>MAAAGASRLLERLLPRHDDFARRHIGPGDKDQREMLQTLGLASIDELIEKTVPANIRLKRPLKMEDPVCENEILATLHAISSKNQIWRSYIGMGYYNCSVPQTILRNLLENSGWITQYTPYQPEVSQGRLESLLNYQTMVCDITGLDMANASLLDEGTAAAEALQLCYRHNKRRKFLVDPRCHPQTIAVVQTRAKYTGVLTELKLPCEMDFSGKDVSGVLFQYPDTEGKVEDFTELVERAHQSGSLACCATDLLALCILRPPGEFGVDIALGSSQRFGVPLGYGGPHAAFFAVRESLVRMMPGRMVGVTRDATGKEVYRLALQTREQHIRRDKATSNICTAQALLANMAAMFAIYHGSHGLEHIARRVHNATLILSEGLKRAGHQLQHDLFFDTLKIQCGCSVKEVLGRAAQRQINFRLFEDGTLGISLDETVNEKDLDDLLWIFGCESSAELVAESMGEECRGIPGSVFKRTSPFLTHQVFNSYHSETNIVRYMKKLENKDISLVHSMIPLGSCTMKLNSSSELAPITWKEFANIHPFVPLDQAQGYQQLFRELEKDLCELTGYDQVCFQPNSGAQGEYAGLATIRAYLNQKGEGHRTVCLIPKSAHGTN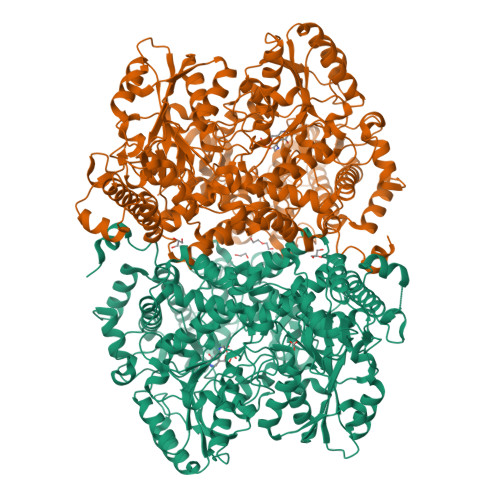PASAHMAGMKIQPVEVDKYGNIDAVHLKAMVDKHKENLAAIMITYPSTNGVFEENISDVCDLIHQHGGQVYLDGANMNAQVGICRPGDFGSDVSHLNLHKTFCIPHGGGGPGMGPIGVKKHLAPFLPNHPVISLKRNEDACPVGTVSAAPWGSSSILPISWAYIKMMGGKGLKQATETAILNANYMAKRLETHYRILFRGARGYVGHEFILDTRPFKKSANIEAVDVAKRLQDYGFHAPTMSWPVAGTLMVEPTESEDKAELDRFCDAMISIRQEIADIEEGRIDPRVNPLKMSPHSLTCVTSSHWDRPYSREVAAFPLPFVKPENKFWPTIARIDDIYGDQHLVCTCPPMEVYESPFSEQKRASSGHHHHHH[4x]>MQAASAFATCLLASVGGNSSAVAFPNQANYSTLVAPYNFDLLTTPSAIVWPQDTQQVAAAVKCAVDSDIKVQPKSGGHNYGNYGSTTGELSVNLDNLQHFSMNETSWTARLGPGNRLGRVTELMYNNGGRHVPHGTTFTVGLGGHATVGGAGAASRMHGLLLDYVEEVEVVLANSSIVRASKSHNEDLFFAVRGAASSVGIVTDFSIRTEPVPVSSVTYSYIWEGTDPAARAEVFLTWQSLLAGGSLPQHMAYDLVATANSMILGGAYFGSQEDFEAFNLSSHFKVAPDVTHIKTYTNFFDFSAAASAQTKAAGIASPSHFYAKSLVFNQQTLIPDDAAEEVFKYLATTKNGTDLYAVTFAALGGAVRDVSASETAFYHRDASYFMFSFGRTSGDLTDTTVQFLDGLSEVLTSGQPDAYYGQYVGNVDPRQPTDEALTGYYGKNLHRLQQIKSAVDPNDVFHNQQSIPPLS[2x]

Sorbicillinoids are yellow secondary metabolites synthesized through an elegant combination of enzymatic and spontaneous biochemical processes. The flavin-dependent monooxygenase SorC and oxidase SorD are crucial in this interplay, enabling the generation of a diverse array of functionally complex sorbicillinoids. SorA and SorB work in tandem to synthesize the hexaketide precursor sorbicillin, while SorC and SorD are involved in the subsequent oxidative processes, including dimerization and oxidation reactions.11,12 Specifically, the monooxygenase SorC catalyzes the oxidative dearomatization of sorbicillin to form (S)-sorbicillinol. The oxidase SorD can then use hydrated sorbicillinol and oxidize it to oxosorbicillinol.

We also obtained the structure of SorD with sorbicillin bound at 3.0 Å. Even though sorbicillin is not the actual substrate — it lacks the hydroxyl group installed by SorC at the C5 position and the additional hydroxyl group from spontaneous water addition at the C6 position — it does mimic hydrated sorbicillinol and binds on the si-face near the N5 locus of FAD in both monomers present in the asymmetric units. Binding analysis using microscale thermophoresis also showed that SorD could bind to sorbicillin with a KD of 1.2 ± 1.6 μM. The electron density was most pronounced in chain B and gave an indication of the preferred binding manner, where the alkyl chain points toward a smaller side pocket lined by hydrophobic residues Ala151, Ala153, Ala252, Ala361, Leu363, Phe385, and Tyr423. Residue Phe387, located on the si-face of FAD, is important in sandwiching the sorbicillin ring between its own aromatic side-chain and the isoalloxazine ring of FAD by π–π stacking interactions. Other polar residues present on the si-face of the FAD in SorD include Tyr80, Asn426, Asp254, and Thr359. The C4–OH of sorbicillin can bond with Tyr80, and its C2–OH can bond with the pyrimidine-2,4-dione part of the FAD. The critical observation is that the C6 carbon of bound sorbicillin is in perfect alignment with flavin N5, should hydrated sorbicillinol be placed in the same position. In this binding orientation and assuming an anti-addition, the 6-hydrogen would point toward the flavin N5 atom for hydride transfer, whereas the 6-OH group would be oriented toward Asp254 and Thr359. The former two residues might function, directly or indirectly through water-mediated interactions, as a catalytic base that promotes alcohol oxidation.>GPGDISHLRVLVAEDNLVNQEVISRMLKQEGITNLTMACNGAKAIDFVKESIENNENFDLIFMDVQMPEVDGLKATKMIRKNLQYNKPIIALTAFADESNVKECLNSGMSGFITKPISKTNIKKVLVEFLSN[4x]

If the HK incorporates a REC domain (REC-1) is denoted as hybrid histidine kinase (hHK), and the first His-Asp phosphotransfer event occurs in the same polypeptide chain. Then, HPt protein containing a phosphorylatable His shuffles the phosphoryl group from the phosphorylatable Asp in the REC-1 domain to the phosphorylatable Asp in the REC domain of an RR (REC-2) in two more phosphotransfer steps. In fungi, the HPt accepts the phosphoryl group from REC-1 domains of various hHKs upstream of the signaling pathway and forwards it downstream to REC-2 domains present in at least two conserved RRs, Ssk1 and Skn7. Also, we have obtained the crystal structures of Ct_HPt alone and in complex with REChHK6 bound to the phosphomimetic BeF3−, as well as the crystal structures of REChHK3 and RECCa_Sln1.

Motivated by our findings and to analyze the Leu-Thr switch in another fungus, we set up crystallization trials with the REC-1 domain of C. albicans (RECCal_Sln1) in the presence of phosphomimetic, either isolated or together with Cal_Ypd1. We obtained crystals for RECCal_Sln1 isolated which contained four molecules in the AU. Again, the molecules did not contain phosphomimetic in the active center, but contained a Mg2+ ion bound stabilized by interactions with the phosphorylatable D1300, residue D1251 in loop β1–α1, main chain carbonyl oxygen of Q1302 in loop β3–α3 and three water molecules. Also, the overall structure was similar to REChHK6 (rmsd of 0.7 Å in 115 residues), but, the loop β4–α4 was ordered and well defined although its conformation slightly differed from REChHK6, as well as the position of α4. The structure of RECCal_Sln1 also provided two interesting features. On one side, the N-terminal H1243 in one molecule was located at a close distance (<6–8 Å) of the phosphorylatable D1300 in another neighbor molecule, however, the distance was not close enough to stabilize the phosphomimetic as it does a catalytic His. On another side, we observed that a Cys in α4 (C1340), which is conserved in the REC-1 domains studied, was connected to a large electron density that may account for a posttranslational modification that we could not identify unambiguously, despite the high resolution of the electron density map (1.5 Å). We also analyzed the active center of RECCal_Sln1 and, as expected, in the absence of phosphomimetic, the OLeu-NAsp+1 distance between Leu in β4 (L1328) and Asp + 1 in β3 corresponds to a hydrogen bond (~3 Å). In this way, all four molecules of RECCal_Sln1 lack the Leu-Thr switch so Thr in β4 (T1329) and Phe in β5 (F1348) were oriented away from the active center. Interestingly, according to the PISA server RECCal_Sln1 also formed two dimers in the crystal (buried area of ~1800 Å2 and ΔGdiss of ~6 kcal/mol).>[2x]MATYPSAKFMECLQYAAFKHRQQRRKDPQETPYVNHVIN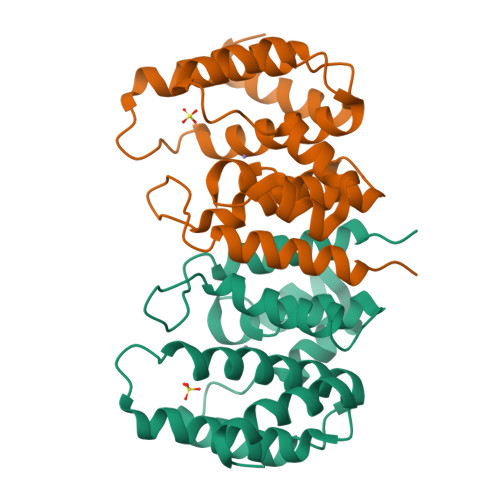VSTILSVEACITDEGVLMAALLHDVVEDTDASFEDVEKLFGPDVCGLVREVTDDKSLEKQERKRLQIENAAKSSCRAKLIKLADKLDNLRDLQVNTPTGWTQERRDQYFVWAKKVVDNLRGTNANLELKLDEIFRQRGLL>GGUUAAAGCCUUAUGGUCGCUACCAUUGCACUCCGGUAGCGUUAAAAGGGAAGACGGGUGAGAAUCCCGCGCAGCCCCCGCUACUGUGAGGGAGGACGAAGCCCUAGUAAGCCACUGCCGAAAGGUGGGAAGGCA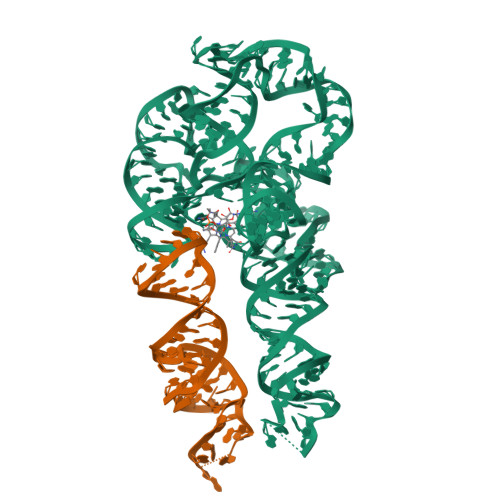GGGUGGAGGAUGAGUCCCGAGCCAGGAGACCUGCCAUAAGGUUUUAGAAGUUCGCCUUCGGGGGGAAGGUGAACA[2x]> LKIQAYFNETADLPCQFANSQNQSLSELVVFWQDQENLVLNEVYLGKEKFDSVHSKYMGRTSFDSDSWTLRLHNLQIKDKGLYQ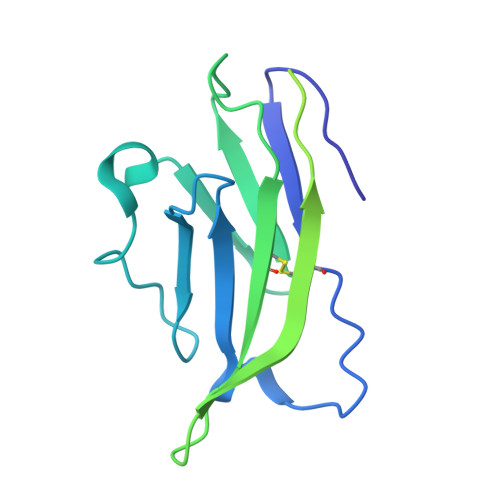CIIHHKKPTGMIRIHQMNSELSVLANFSQPEIVPISNITENVYINLTCSSIHGYPEPKKMSVLLRTKNSTIEYDGVMQKSQDNVTELYDVSISLSVSFPDVTSNMTIFCILETDKTRLLSSPFSIELED> GPHMKSPSAQELKEQGNRLFVGRKYPEAAACYGRAITRNPLVAVYYTNRALCYLKMQQPEQALADCRRALELDGQSVKAHFFLGQCQLEMESYDEAIANLQRAYSLAKEQRLNF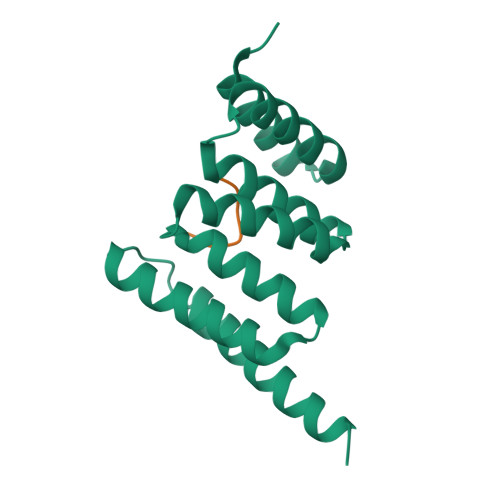GDDIPSALRIAKKKRWNSIEERR;> SPHNPISDVD> GDRVADVIESSIGDSVSRALTHALPAPTGQNTQVSSHRLDTGKVPALQAA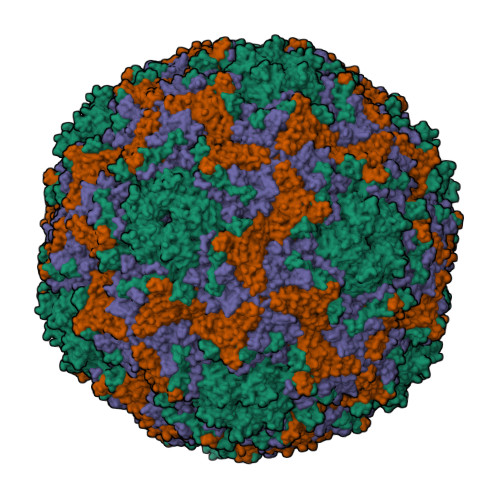EIGASSNASDESMIETRCVLNSHSTAETTLDSFFSRAGLVGEIDLPLKGTTNPNGYANWDIDITGYAQMRRKVELFTYMRFDAEFTFVACTPTGEVVPQLLQYMFVPPGAPKPDSRESLAWQTATNPSVFVKLSDPPAQVSVPFMSPASAYQWFYDGYPTFGEHKQEKDLEYGAMPNNMMGTFSVRTVGTSKSKYPLVVRIYMRMKHVRAWIPRPMRNQNYLFKANPNYAGNSIKPTGASRTAITTL;> SDRVAQLTIGNSTITTQEAANIIVGYGEWPSYCSDSDATAVDKPTRPDVSVNRFYTLDTKLWEKSSKGWYWKFPDVLTETGVFGQNAQFHYLYRSGFCIHVQCNASKFHQGALLVAVLPEYVIGTVAGGTGTEDTHPPYKQTQPGADGFELQHPYVLDAGIPISQLTVCPHQWINLRTNNCATIIVPYINALPFDSALNHCNFGLLVVPISPLDYDQGATPVIPITITLAPMCSEFAGLRQAVTQ;> GFPTELKPGTNQFLTTDDGVSAPILPNFHPTPCIHIPGEVRNLLELCQVETILEVNNVPTNATSLMERLRFPVSAQAGKGELCAVFRADPGRNGPWQSTLLGQLCGYYTQWSGSLEVTFMFTGSFMATGKMLIAYTPPGGPLPKDRATAMLGTHVIWDFGLQSSVTLVIPWISNTHYRAHARDGVFDYYTTGLVSIWYQTNYVVPIGAPNTAYIIALAAAQKNFTMKLCKDASDILQTGTIQ;> SHENSNSATEGSTINYTTINYYKDSYAATAGKQSLKQDPDKFANPVKDIFTEMAAPLK>[2x]MSEFHSEISTLSPAPLWQFFDKICSIPHPSKHEEALAQYIVTWATEQGFDVRRDPTGNVFIKKPATPGMENKKGVVLQAHIDMVPQKNEDTDHDFTQDPIQPYIDGEWVTAKGTTLGADNGIGMASCLAV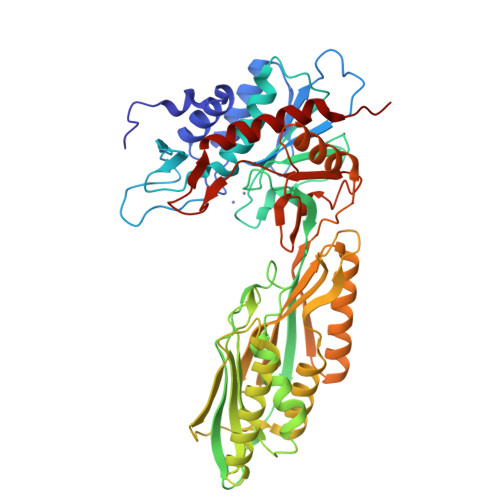LASKEIKHGPIEVLLTIDEEAGMTGAFGLEAGWLKGDILLNTDSEQEGEVYMGCAGGIDGAMTFDITRDAIPAGFITRQLTLKGLKGGHSGCDIHTGRGNANKLIGRFLAGHAQELDLRLVEFRGGSLRNAIPREAFVTVALPAENQDKLAELFNYYTELLKTELGKIETDIVTFNEEVATDAQVFAIADQQRFIAALNACPNGVMRMSDEVEGVVETSLNVGVITTEENKVTVLCLIRSLIDSGRSQVEGMLQSVAELAGAQIEFSGAYPGWKPDADSEIMAIFRDMYEGIYGHKPNIMVIHAGLECGLFKEPYPNMDMVSFGPTIKFPHSPDEKVKIDTVQLFWDQMVALLEAIPEKA>MNVARIGIGQLCSSSNLKQNLEVVKSLIKKALDQDVKVLFFPEATDYLSRNAEHSKKLASQTPEFISELQSAICQLTKAAGKPIDISIGIHMPPSEVNTKNGDSRVKNVLLYINSNGEILQKYQKLHLFDVDVPNGPILKESNSVQPGSEIPSIINTPVGKLGSCICYDIRFPELSLKLRSKGAQILCFPSAFTMK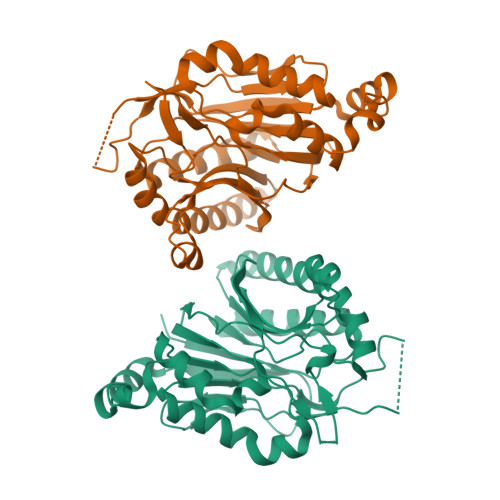TGEAHWELLGRARAIDTQSFVVMPAQQGEHDVYADEKPSDESAVKRISWGHSMIIDPWGRILSAADLTTHDPQLIIADLDIEAQDKIRRDMPLWAQRRRDIFGDFV[4x]>[2x]GKTNDWLDFDQLAEEKVRDALKPPSMYKVILVND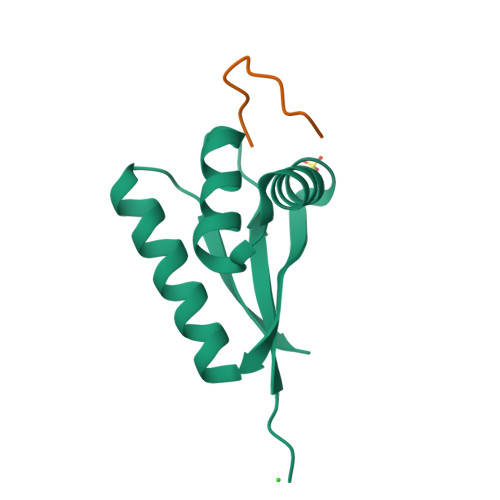DYTPMEFVIDVLQKFFSYDVERATQLMLAVHYQGKAICGVFTAEVAETKVAMVNKYARENEHPLLCTLEKA;>FRSKGEELFT[2x]> AQYEDGKQYTTLEKPVAGAPQVLEFFSFFCPHCYQFEEVLHISDNVKKKLPEGVKMTKYHVNFMGGDLGKDLTQAWAVAMALGVEDKVTVPLFEGVQKTQTIRSASDIRDVFINAGIKGEEYDAAWNSFVVKSLVAQQEKAAA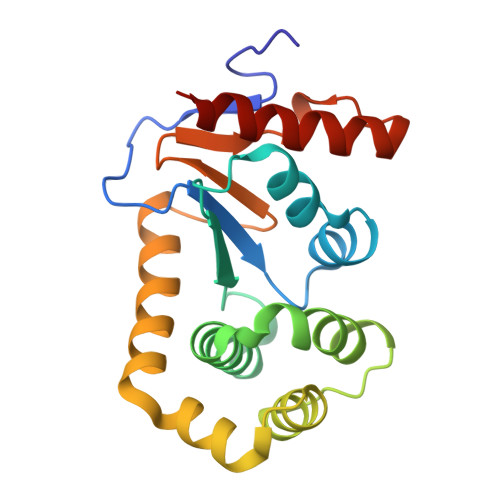DVQLRGVPAMFVNGKYQLNPQGMDTSNMDVFVQQYADTVKYLSEEK S-methyl methanesulfonothioate 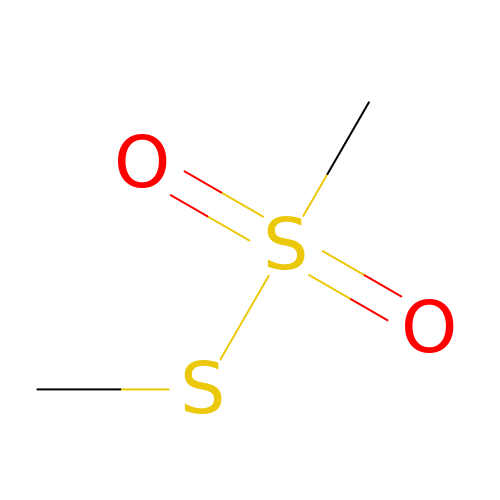| C2 H6 O2 S2 | XYONNSVDNIRXKZ-UHFFFAOYSA-N>GPGEIRPTIGQQMETGDQRFGDLVFRQLAPNVWQHTSYLDMPGFGAVASNGLIVRDGGRVLVVDTAWTDDQTAQILNWIKQEINLPVALAVVTHAHQDKMGGMDALHAAGIATYANALSNQLAPQEGMVAAQHSLTFAANGWVEPATAPNFG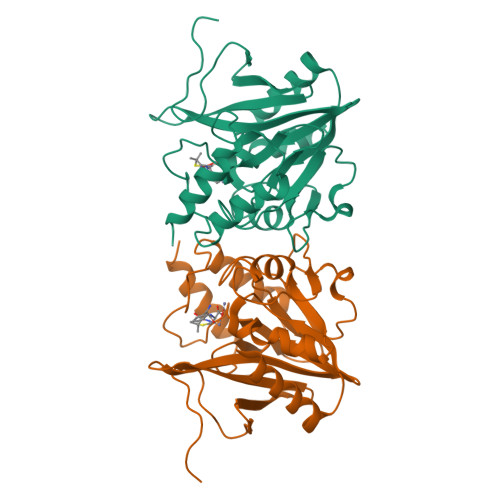PLKVFYPGPGHTSDNITVGIDGTDIAFGGCLIKDSKAKSLGNLGDADTEHYAASARAFGAAFPKASMIVMSHSAPDSRAAITHTARMADKLR[2x]>[8x]GPLGSDADKNDPAGKDQQVNVGETPKAEDSIGNLPDLPKGTTVAFETPVDTATPGDKPAKVVVTYPDGSKDTVDVTVKVVDPRTDADKNDPAGKDQQVNVG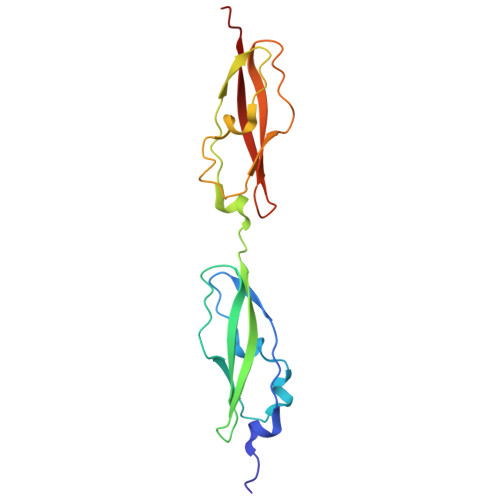ETPKAEDSIGNLPDLPKGTTVAFETPVDTATPGDKPAKVVVTYPDGSKDTVDVTVKVVDPRT> EERNDWHFNIGAMYEIENVEGYGEDMDGLAEPSVYFNAANGPWRIALAYYQEGPVDYSAGKRGTWFDRPELEVHYQFLENDDFSFGLTGGFRNYGYHYVDEPGK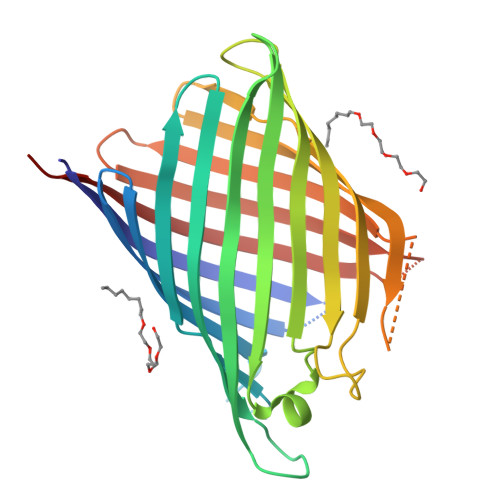DTANMQRWKIAPDWDVKLTDDLRFNGWLSMYKFANDLNTTGYADTRVETETGLQYTFNETVALRVNYYLERGFNMDDSRNNGEFSTQEIRAYLPLTLGNHSVTPYTRIGLDRWSNWDWQDDIEREGHDFNRVGLFYGYDFQNGLSVSLEYAFEWQDHDEGDSDKFHYAGVGVNYSFHHHHHH>GAMAGKAVPMQSKKKIFKPEELRQALMPTLEALYRQD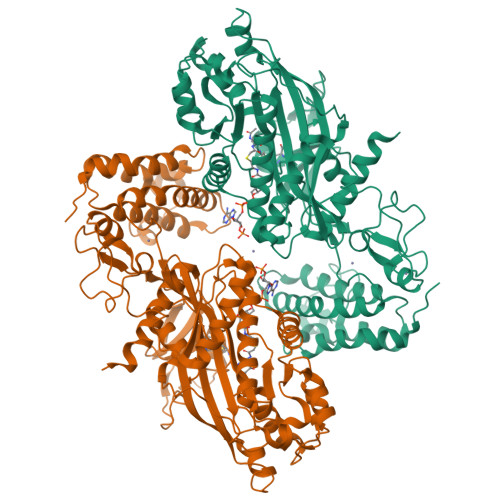PESLPFRQPVDPQLLGIPDYFDIVKSPMDLSTIKRKLDTGQYQEPWQYVDDIWLMFNNAWLYNRKTSRVYKYCSKLSEVFEQEIDPVMQSLGYCCGRKLEFSPQTLCCYGKQLCTIPRDATYYSYQNRYHFCEKCFNEIQGESVSLGDDPSQPQTTINKEQFSKRKNDTLDPELFVECTECGRKMHQICVLHHEIIWPAGFVCDGCLKKSARTRKENKFSAKRLPSTRLGTFLENRVNDFLRRQNHPESGEVTVRVVHASDKTVEVKPGMKARFVDSGEMAESFPYRTKALFAFEEIDGVDLCFFGMHVQEYGSDCPPPNQRRVYISYLDSVHFFRPKCLRTAVYHEILIGYLEYVKKLGYTTGHIWACPPSEGDDYIFHCHPPDQKIPKPKRLQEWFKKMLDKAVSERIVHDYKDIFKQATEDRLTSAKELPYFEGDFWPNVLEESIKESGGSGSQKLYATMEKHKEVFFVIRLIAGPAANSLPPIVDPDPLIPCDLMDGRDAFLTLARDKHLEFSSLRRAQWSTMCMLVELHTQSQDRF[2x]>[2x]GLTEEQRMMIRELMDAQMKTFDTTFSHFKNFRLPGVLSSGCELPESLQAPSREEAAKWSQVRKDLCSLKVSLQLRGEDGSVWNYKPPADSGGKEIFS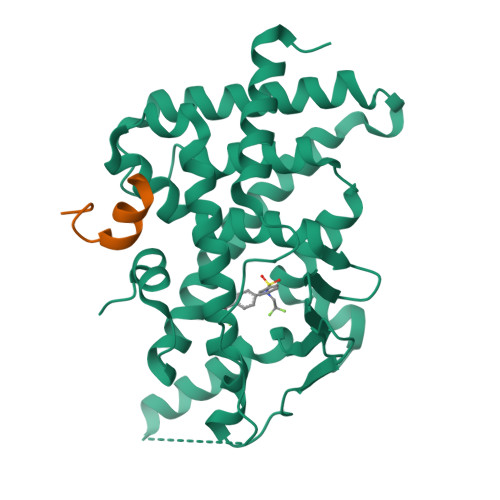LLPHMADMSTYMFKGIISFAKVISYFRDLPIEDQISLLKGAAFELSQLRFNTVFNAETGTWECGRLSYCLEDTAGGFQQLLLEPMLKFHYMLKKLQLHEEEYVLMQAISLFSPDRPGVLQHRVVDQLQEQFAITLKSYIECNRPQPAHRFLFLKIMAMLTELRSINAQHTQRLLRIQDIHPFATPLMQELFGITGS;>[2x]SLTERHKILHRLLQE> GSTPTINIPASPFMQKLGFGTGVNVYLMKRSPRGLSHSPWAVKKINPICNDHYRSVYQKRLMDEAKILKSLHHPNIVGYRAFTEANDGSLCLAMEYGGEKSLNDLIEERYKASQDPFPAAIILKVALNMARGLKYLHQEKKLLHGDIKSSNVVIKGDFETIKICDVGVSLPLDENMEVTDPEACYIGTEPWKPKEAVEENGVITDKADIFAFGLTLWEMMTLSIPHINLSNDDDDEDKTFDESDFDDEAYYAALGTRPPINMEELDESYQKVIELFSVCTNEDPKDRPSAAHIVEALETA;> GSVLCSTPTINIPASPFMQKLGFGTGVNVYLMKRSPRGLSHSPWAVKKINPICNDHYRSVYQKRLMDEAKILKSLHHPNIVGYRAFTEANDGSLCLAMEYGGEKSLNDLIEERYKASQDPFPAA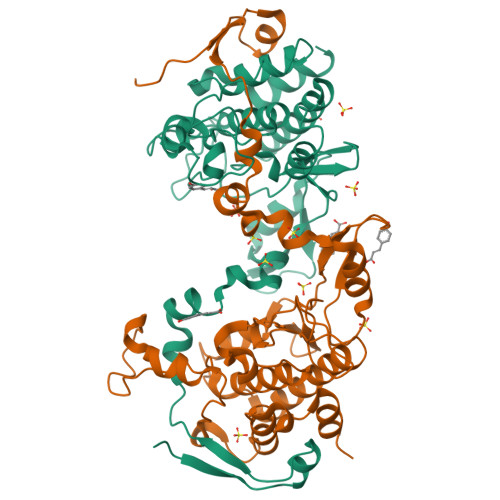IILKVALNMARGLKYLHQEKKLLHGDIKSSNVVIKGDFETIKICDVGVSLPLDENMEVTDPEACYIGTEPWKPKEAVEENGVITDKADIFAFGLTLWEMMTLSIPHINLSNDDDDEDKTFDESDFDDEAYYAALGTRPPINMEELDESYQKVIELFSVCTNEDPKDRPSAAHIVEALEAA> GPPQFKPLKISVDPEIPAPPAI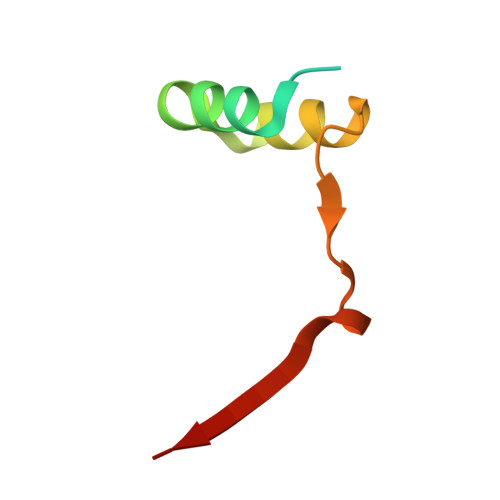ADLLASVDSEEVREYCKKKGWIVEVPVTATTLERNVS>[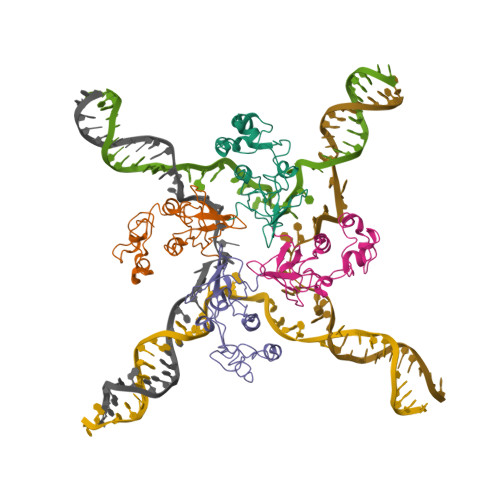4x]MIRYLRGLVLKKEAGGFVLLAGGVGFFLQAPTPFLQALEEGKEVGVHTHLLLKEEGLSLYGFPDEENLALFELLLSVSGVGPKVALALLSALPPRLLARALLEGDARLLTSASGVGRRLAERIALELKGKVPPHLLAGEK(2S,3R,4S,5S)-2-(acetylamino)-5-carboxy-3,4-dihydroxypiperidinium 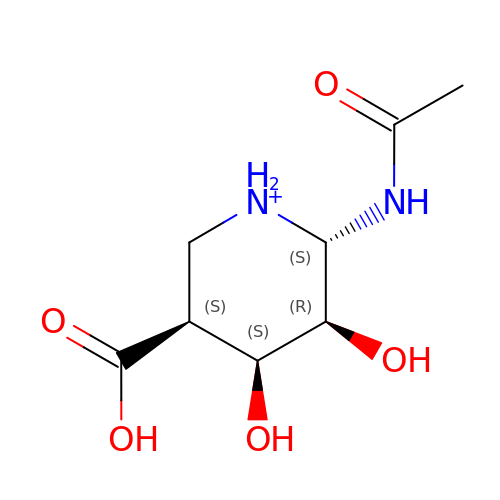| C8 H15 N2 O5 | DQTKLICLJUKNCG-ZTYPAOSTSA-O In bacteria, two distinct G3P acyltransferases (GPATs), PlsB and PlsY, catalyse the committed step. By contrast, the recently identified membrane-integral PlsY exists exclusively and ubiquitously in bacteria, and uses an unusual acyl donor, namely the acyl-phosphate (acylP), representing a unique class of acyltransferase. PlsY acylates G3P using acylP, forming lysoPA and inorganic phosphate (Pi). The overall shape of aaPlsY resembles a funnel composed of three tilted helices (α1–3) sitting in a cup composed of seven TMHs.

As shown in the aaPlsYlysoPA structure, the phosphate group of lysoPA is located in the phosphate clamp, which is the same site for Pi/3. Thus, the path for Pi release is blocked by lysoPA, suggesting that the lysoPA liberation is requisite for Pi release. Our structures show that lysoPA interacts with all G3P-binding residues, and forms three additional H-bonds to backbone amides of Ala40 and Thr41, and the Thr41 hydroxyl. Furthermore, its hydrocarbon tail is anchored in the hydrophobic groove as seen for 16 : 0-P binding. Therefore, lysoPA should bind to PlsY with much higher affinity than does for G3P, featuring a competitive inhibitor. The release of the product inhibitor is probably driven by high concentrations of the substrates. In addition, the exiting Pi along the Pi-release path might aid the lysoPA clearance by electro-repulsion and competing for the phosphate clamp site.

>[2x]MGSALFLVIFAYLLGSITFGEVIAKLKGVDLRNVGSGNVGATNVTRALGKKYGVLVFFLDFLKGFIPALIAVKSFGIDSWVLTFTGLASVLGHMYPVFFGFKGGKGVATALGVVFAVSPSVALFSFLVWLGIFLWKRYVSLASITATISAFLFLFVAGYPVNVLFMAIVIGALIIYRHRENINRLLTGREHRFGTLEVLFQ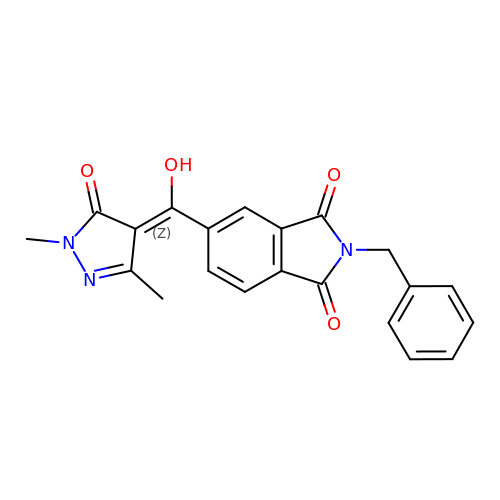5-[(~{Z})-(1,3-dimethyl-5-oxidanylidene-pyrazol-4-ylidene)-oxidanyl-methyl]-2-(phenylmethyl)isoindole-1,3-dione | C21 H17 N3 O4 | ZWUMMDOCWXLHBD-ZCXUNETKSA-N>[2x]AHNNENVSGISAYLLGLIIGDGGLYKLKYKGNRSEYRVVITQKSENLIKQHIAPLMQFLIDELNVKSKIQI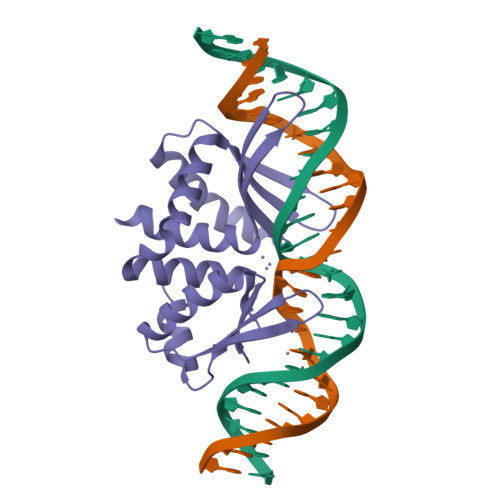VKGDTRYELRVSSKKLYYYFANMLERIRLFNMREQIAFIKGLYVAEGDKTLKRLRIWNKNKALLEIVSRWLNNLGVRNTIHLDDHRHGVYVLNISLRDRIKFVHTILSSHLNPLPPEAAALEHHHHHH;> AHNNEEVSGISAYLLGLIIGDGGLYKLKYKGNRSEYRVVITQKSENLIKQHIAPLMQFLIDELNVKSKIQIVKGDTRYELRVSSKKLYYYFANMLERIRLFNMREQIAFIKGLYVAEGDKTLKRLRIWNKNKALLEIVSRWLNNLGVRNTIHLDDHRHGVYVLNISLRDRIKFVHTILSSHLNPLPPEAAALEHHHHHH> FPTDDDDKIVGGYTCAANSIPYQVSLNSGSHFC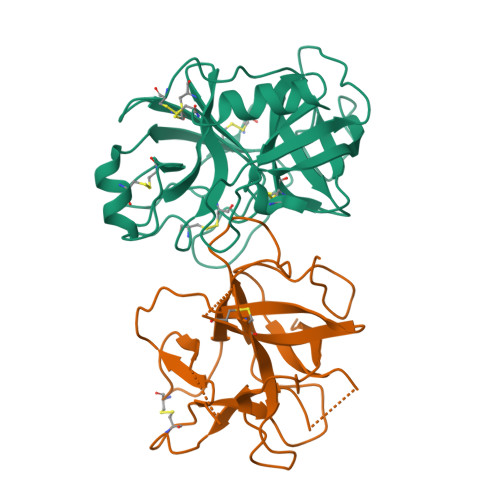GGSLINSQWVVSAAHCYKSRIQVRLGEHNIDVLEGNEQFINAAKIITHPNFNGNTLDNDIMLIKLSSPATLNSRVATVSLPRSCAAAGTECLISGWGNTKSSGSSYPSLLQCLKAPVLSDSSCKSSYPGQITGNMICVGFLEGGKDSCQGDSGGPVVCNGQLQGIVSWGYGCAQKNKPGVYTKVCNYVNWIQQTIAAN;> DYTVHDTDGKPVLNNAGQYYILPAKQGKGGGLGLSNDDDGNCPLTVSQTPIDIPIGLPVRFSSRARISHITTALSLNIEFTIAPACAPKPARWRIFDEQSSEKGYTPVKISDDFSSAAPFQIKKFEEDYKLVYCSKSESGERKCVDLGIKIDNEKNRRLVLKEGDPFKVKFKKVDEESSEEWSIV> GMSNNMQTVRESYEAFHRRDLPGVLAALAPDVRWTHPDGMSPYGLGGTKHGHDEVIAFIRHVPTHIAEMRLAPDEFIESGERIVVLGTRRV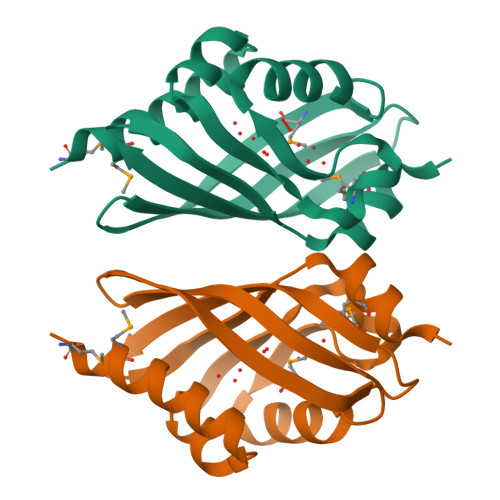TAVNGRSATLKFVHVWRFENGRAVTFEDHFDTAEMIRLITA>[16x]DGGDSGDTGNGWHGAQMDFARDMSYGDYLGLDQILSAQHPLSPDHNEMLFIVQHQTTELWMKLMLHELRAARDGVKSDQLQPAFKMLARVSRIMDQLVQAWNV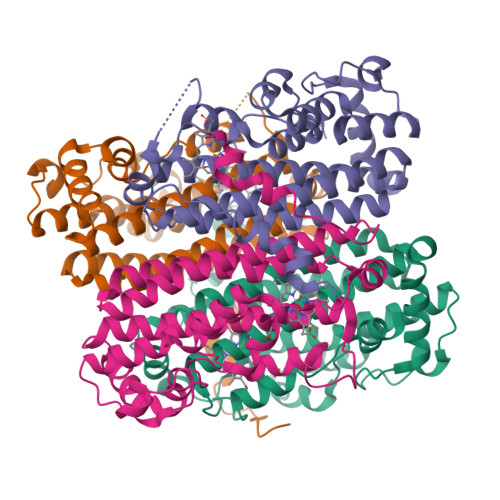LATMTPPEYSAMRPYLGASSGFQSYQYREIEFILGNKNAAMLRPHAHRPEHLELVETALHTPSMYDEAIRLMARRGFQIDPEVVERDWTQPTQYNASVEAAWLEVYRNPSAHWELYELGEKFVDLEDAFRQWRFRHVTTVERVIGFKRGTGGTEGVSYLRRMLDVVLFPELWKLRTDL>[4x]MKKTKIVCTIGPKTESEEMLAKMLDAGMNVMRLNFSHGDYAEHGQRIQNLRNVMSKTGKTAAILLDTKGPEIRTMKLEGGNDVSLKAGQTFTFTTDKSVIGNS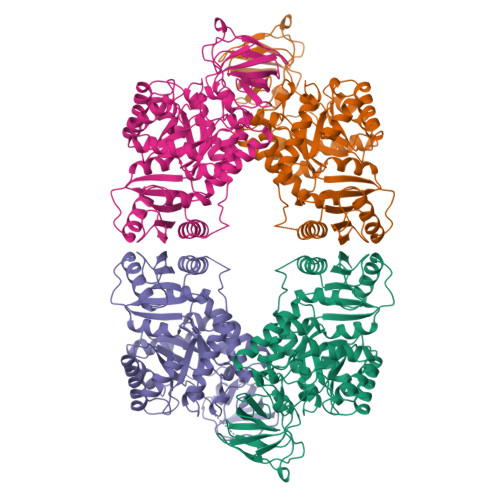EMVAVTYEGFTTDLSVGNTVLVDDGLIGMEVTAIEGNKVICKVLNNGDLGENKGVNLPGVSIALPALAEKDKQDLIFGCEQGVDFVAASFIRKRSDVIEIREHLKAHGGENIHIISKIENQEGLNNFDEILEASDGIMVARGDLGVEIPVEEVIFAQKMMIEKCIRARKVVITATMMLDSMIKNPRPTRAEAGDVANAILDGTDAVMLSGESAKGKYPLEAVSIMATICERTDRVMNSRLEFNNDNRKLRITEAVCRGAVETAEKLDAPLIVVATQGGKSARAVRKYFPDATILALTTNEKTAHQLVLSKGVVPQLVKEITSTDDFYRLGKELALQSGLAHKGDVVVMVSGALVPSGTTNTASVHVL> GSMSSERVLSYAPAFKSFLDTSFFQELSRLKLDVLKLDSTCQPLTVNLDLHNIPKSADQVPLFLTNRSFEKHNNKRTNEVPLQGSIFNFNVLDEFKNLDKQLFLHQRALECWEDGIKDINKCVSFVIISFADLKKYRFYYWLGVPCFQRPSSTVLHVRPEPSLKGLFSKCQKWFDVNYSKWVCILDADDEIVNYDKCIIRKTKVLAIRDTSTMENVPSALTKNFLSVLQYDVPDLIDFKLLIIRQNEGSFALNATFASIDPQSSSSNPDMKVSGWERNVQGKLAPRV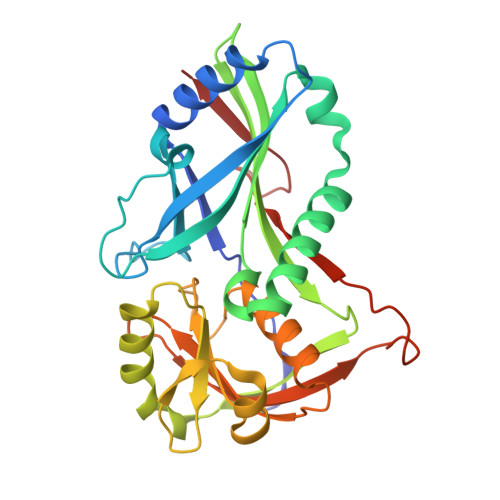VDLS> MAATTESVKADAAEAPLLNKKNIIAGASLYLVFYAWVRWYEGVYGWSAGLDSFAPEFETYWMNFLYIEMVLEVLTASVLWGYIWKSRDRKVMSITPREELRRHFTHWTWLMMYGIAIYFGASYFTEQDGTWHQTIVRDTDFTPSHIIEFYLSYPIYIITGGASFLYAKTRLPTYQQGLSLQYLVVVVGPF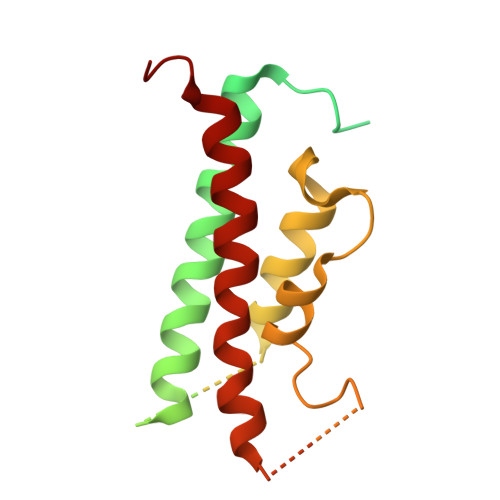MILPNVGLNEWGHTFWFMEELFVAPLHYGFVFFGWSALGVLGVINIELGALSKLLKKDLA(2R,3R)-4-[(2R)-2-(3-chlorophenyl)pyrrolidin-1-yl]-2,3-dihydroxy-4-oxo-N-[(5-{[2-(trifluoromethyl)-1H-benzimidazol-1-yl]methyl}thiophen-2-yl)methyl]butanamide 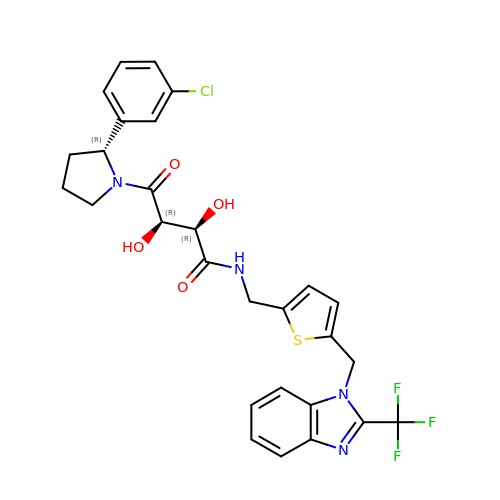| C28 H26 Cl F3 N4 O4 S | JSNHRUZOJTYCCL-GMKZXUHWSA-N>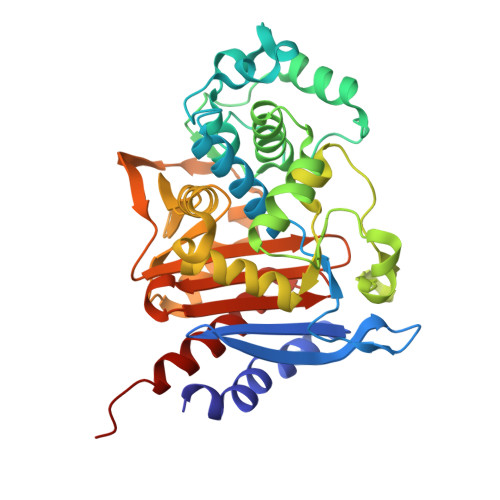 GEAPADRLKALVDAAVQPVMKANDIPGLAVAISLKGEPHYFSYGLASKEDGRRVTPETLFEIGSVSKTFTATLAGYALTQDKMRLDDRASQHWPALQGSRFDGISLLDLATYTAGGLPLQFPDSVQKDQAQIRDYYRQWQPTYAPGSQRLYSNPSIGLFGYLAARSLGQPFERLMEQQVFPALGLEQTHLDVPEAALAQYAQGYGKDDRPLRVGPGPLDAEGYGVKTSAADLLRFVDANLHPERLDRPWAQALDATHRGYYKVGDMTQGLGWEAYDWPISLKRLQAGNSTPMALQPHRIARLPAPQALEGQRLLNKTGSTNGFGAYVAFVPGRDLGLVILANRNYPNAERVKIAYAILSGLEQQGKVPLKR> AQSLSFSFTKFDPNQEDLIFQGHATSTNNVLQVTKLD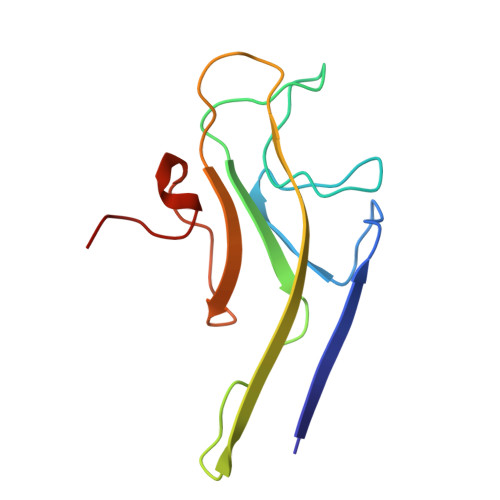SAGNPVSSSAGRVLYSAPLRLWEDSAVLTSFDTIINFEISTPYTSRIADGLAFFIAPPDSVISYHGGFLGLFPNAN>[5x]MTVTYTARVANARFGGFSQLLLLWRGSIYKLLWRELLCFLGFYMALSAAYRFVLTEGQKRYFEKLVIYCDQYASLIPVSFVLGFYVTLVVNRWWSQYLCMPLPDALMCVVAGTVHGRDDRGRLY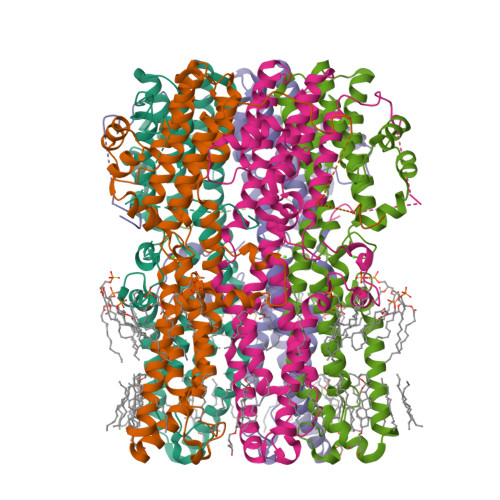RRTLMRYAGLSAVLILRSVSTAVFKRFPTIDHVVEAGFMTREERKKFENLNSSYNKYWVPCVWFSNLAAQARREGRIRDNSALKLLLEELNVFRGKCGMLFHYDWISVPLVYTQVVTIALYSYFLACLIGRQFLDPAQGYKDHDLDLCVPIFTLLQFFFYAGWLKVAEQLINPFGEDDDDFETNFLIDRNFQVSMLAVDEMYDDLAVLEKDLYWDAAEARAPYTAATVFQLRQPSFQGSTFDITLAKEDMQFQRLDGLDGPMGEAPGDFLQRLLPAGAGMVA3-{[(E)-AMINO(HYDROXYIMINO)METHYL]AMINO}ALANINE | C4 H10 N4 O3 | 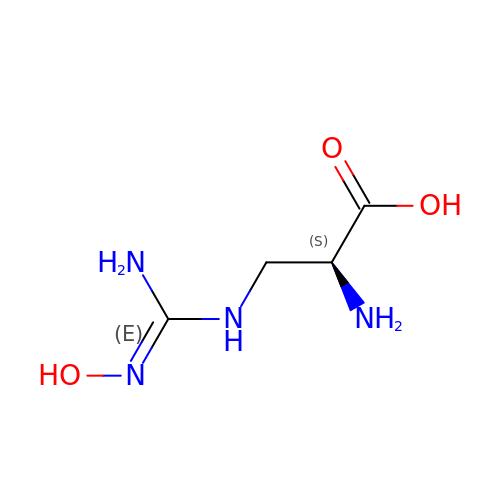RPHCSGPGZUWMRV-REOHCLBHSA-N N-[2-(dimethylamino)ethyl]-N-[[4-[[4-methyl-3-[(4-pyridin-3-ylpyrimidin-2-yl)amino]phenyl]carbamoyl]phenyl]methyl]pyridine-3-carboxamide 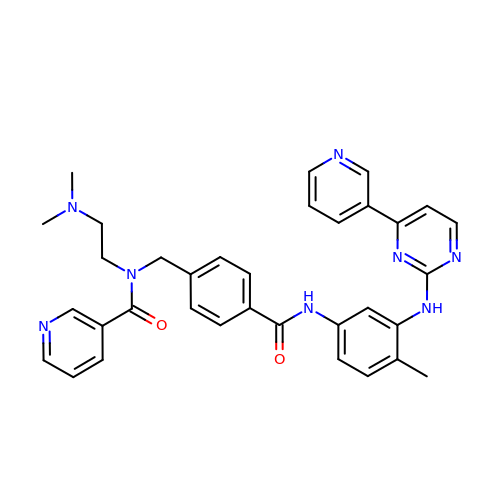| C34 H34 N8 O2 | NWVOHJOHQOHBMB-UHFFFAOYSA-N> MGSSHHHHHHSSGRENLYFQGSKELLRLQKELKDIENENVQEIDAHIKDSNFFEWVGFIKGPEGTPYEGGHFTLAITIPNDYPYNPPKIKFVTKIWHPNI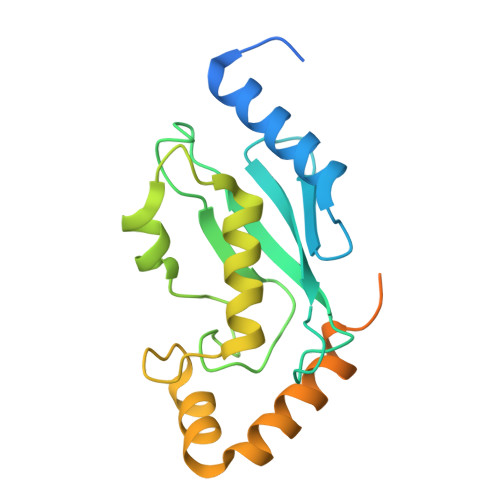SSQTGAICLDVLKNEWSPALTIRTALLSIQALLSDPQPDDPQDAEVAKMYKENHALFVKTASVWTKTFATGPKEEPREVIIKKITEMGFSEDQAKNALIKANWNETLALNTLLENS CARDIOLIPIN | C58 H120 O17 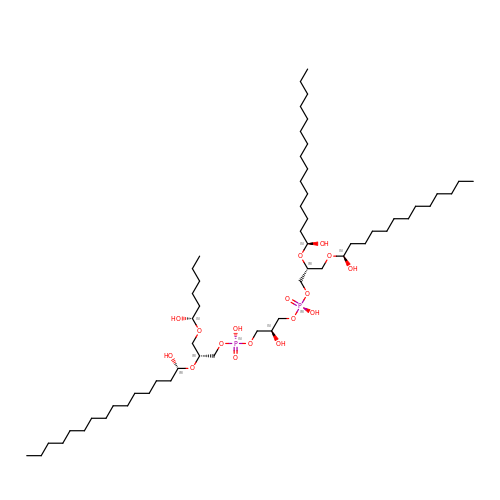P2 | GKRASOJOCMJQMF-DUXRJKJQSA-N>SNAMALKKPGSLTI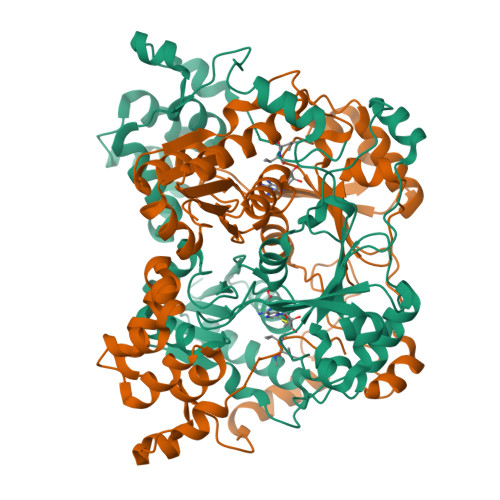AGSGIASIGHITLETLALIKEADKIFYAVTDPATECYIQENSRGDHFDLTTFYDTNKKRYESYVQMSEVMLRDVRAGRNVLGIFYGHPGVFVAPSHRAIAIAREEGFQAKMLPGISAEDYMFADLGFDPSTYGCMTQEATELLVRNKKLDPSIHNIIWQVGSVGVDTMVFDNGKFHLLVERLEKDFGLDHKIQHYIGAILPQSVTVKDTFAIRDLRKEEVLKQFTTTSTFYVPPRTPAPIDPKAVQALGLPATVTKGAQDWTGFQSVSPAYGPDEMRAVAALDSFVPSQEKAVVHASRAMQSLMVDLALRPALLEQYKADPVAFANTRNGLTAQEKFALGLKKPGPIFVVMRQLPSAIASGQEPSQEEIARADDATALALVVVIVQ[4x]The human heterodimeric amino acid transporter 4F2hc-LAT2 is a membrane protein complex that mediates transport of certain amino acids and derivatives thereof across the plasma membrane. While CATs are N-glycosylated, LATs are not but they associate with type-II membrane N-glycoproteins from the SLC3 family, i.e., either with 4F2hc (SLC3A2; CD98hc) or with rBAT (SLC3A1), to form heterodimeric amino acid transporters (HATs). Light chains are polytopic membrane proteins with both termini located on the cytoplasmic side, which function as the substrate transporters. Anticalins are composed of a central eight-stranded antiparallel β-barrel backed by an extended strand and an α-helical segment.

We overexpressed the human HAT 4F2hc-LAT2 in the yeast Pichia pastoris, purified the protein in the presence of detergent and solved its structure by cryo-EM at 3.2 Å resolution after complex formation with the anticalin D11vs produced in E. coli. The structure of 4F2hc-LAT2 with the bound anticalin D11vs was captured in the inward-open conformation as evidenced by the large cavity (red asterisk) facing the cytoplasm. LAT2 is covalently linked to 4F2hc via a disulfide bridge. The 4F2hc-ED sits on top of LAT2 and forms a complex with D11vs. The overall resolution of the final cryo-EM 3D density map calculated from differently oriented 4F2hc-LAT2::D11vs complex particles was estimated to 3.2 Å according to the gold standard Fourier shell correlation (FSC) cut-off criterion of 0.14339,40. Local resolution analysis of the map indicated that the highest resolution features (2.8–3.0 Å) were located in the substrate binding region of LAT2 (S) and in the interface region between 4F2hc-ED and D11vs (I) (labels S and I in Fig. 2d). The high local resolution and quality of the cryo-EM density permitted modelling of D11vs with high confidence. Interestingly, three defined densities were found in the substrate binding pocket, which we attributed to water molecules: H2O-1, H2O-2 and H2O-3. In our structure, H2O-1 is 3.9 Å apart from the amide nitrogen atom of G57 and could thus correspond to the location of one oxygen atom of the carboxyl group in an amino acid substrate. In order to support the existence of the three observed water molecules in the substrate binding pocket of LAT2, a set of four all-atom molecular dynamics (MD) simulations of the 4F2hc-LAT2::D11vs complex was performed under near physiological conditions. The persistent presence of water molecules at all three positions was confirmed with occupancies of H2O-1: 59.3 ± 4.3%, H2O-2: 65.1 ± 4.5% and H2O-3: 52.7 ± 11.4%. No significant structural differences were observed between our structure and previously reported 4F2hc-ED and 4F2hc-LAT2 structures.

> TMAHHHHHHHHHGIEGRMSQDTEVDMKEVELNELEPEKQPMNAASGAAMSLAGAEKNGLVKIKVAEDEAEAAAAAKFTGLSKEELLKVAGSPGWVRTRWALLLLFWLGWLGMLAGAVVIIVRAPRCRELPAQKWWHTGALYRIGDLQAFQGHGAGNLAGLKGRLDYLSSLKVKGLVLGPIHKNQKDDVAQTDLLQIDPNFGSKEDFDSLLQSAKKKSIRVILDLTPNYRGENSWFSTQVDTVATKVKDALEFWLQAGVDGFQVRDIENLKDASSFLAEWQNITKGFSEDRLLIAGTNSSDLQQILSLLESNKDLLLTSSYLSDSGSTGEHTKSLVTQYLNATGNRWCSWSLSQARLLTSFLPAQLLRLYQLMLFTLPGTPVFSYGDEIGLDAAALPGQPMEAPVMLWDESSFPDIPGAVSANMTVKGQSEDPGSLLSLFRRLSDQRSKERSLLHGDFHAFSAGPGLFSYIRHWDQNERFLVVLNFGDVGLSAGLQASDLPASASLPAKADLLLSTQPGREEGSPLELERLKLEPHEGLLLRFPYAA;> MAWSHPQFEKIEGRMEEGARHRNNTEKKHPGGGESDASPEAGSGGGGVALKKEIGLVSACGIIVGNIIGSGIFVSPKGVLENAGSVGLALIVWIVTGFITVVGALCYAELGVTIPKSGGDYSYVKDIFGGLAGFLRLWIAVLVIYPTNQAVIALTFSNYVLQPLFPTCFPPESGLRLLAAICLLLLTWVNCSSVRWATRVQDIFTAGKLLALALIIIMGIVQICKGEYFWLEPKNAFENFQEPDIGLVALAFLQGSFAYGGWNFLNYVTEELVDPYKNLPRAIFISIPLVTFVYVFANVAYVTAMSPQELLASNAVAVTFGEKLLGVMAWIMPISVALSTFGGVNGSLFTSSRLFFAGAREGHLPSVLAMIHVKRCTPIPALLFTCISTLLMLVTSDMYTLINYVGFINYLFYGVTVAGQIVLRWKKPDIPRPIKINLLFPIIYLLFWAFLLVFSLWSEPVVCGIGLAIMLTGVPVYFLGVYWQHKPKCFSDFIELLTLVSQKMCVVVYPEVERGSGTEEANEDMEEQQQPMYQPTPTKDKDVAGQPQP;> QDSTSDLIPAPPLSKVPLQQNFQDNQFHGKWYVVGRAGNTGLREDKDPGKMFATIYELKEDKSYNVTYVWSGQKKCMYSIVTFVPGSQPGEFTLGNIKSAPGRTSWLVRVVSTNYNQHAMVFFKSVTQNREGFAITLYGRTKELTSELKENFIRFSKSLGLPENHIVFPVPIDQCIDGSAWSHPQFEK>[2x]SGEPRTRAEARPWVDEDLKDSSDLHQAEEDADEWQESEENVEHIPFSHNHYPEKEMVKRSQEFYELLNKRRSVRFISNEQVPMEVIDNVIRTAGTAPSGAHTEPWTFVVVKDPDVKHKIRKIIEEEEEINYMKRMGHRWVTDL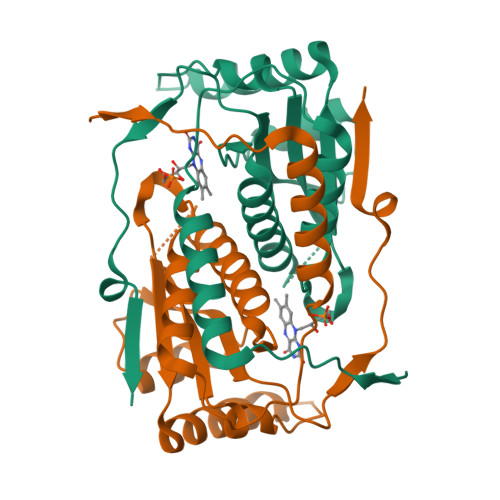KKLRTNWIKEYLDTAPILILIFKQVHGFAANGKKKVHYYNEISVSIACGILLAALQNAGLVTVTTTPLNCGPRLRVLLGRPAHEKLLMLLPVGYPSKEATVPDLKRKPLDQIMVTVHHHHHH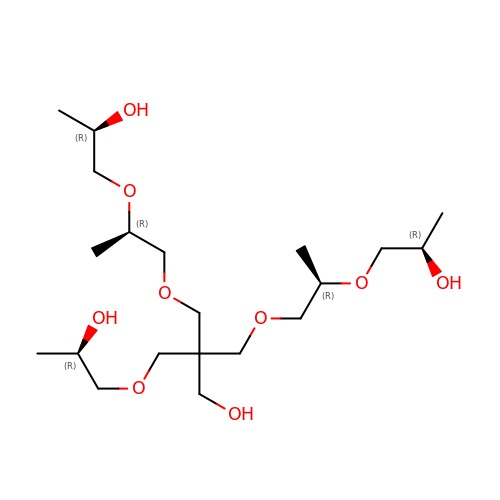(2R,5R,13R,16R)-9-(hydroxymethyl)-9-{[(2R)-2-hydroxypropoxy]methyl}-5,13-dimethyl-4,7,11,14-tetraoxaheptadecane-2,16-diol | C20 H42 O9 | XAZUABIGWFVOAV-FVVUREQNSA-N> MIQKMALDEFDSLGDKVIEGYQLTDNDLRTLLSLESKEGLERLYSAARKVRDHYFGNRVFLNCFIYFSTYCKNQCSFCYYNCRNEINRYRLTMEEIKETCKTLKGAGFHMVDLTMGEDPYYYEDPNRFVEL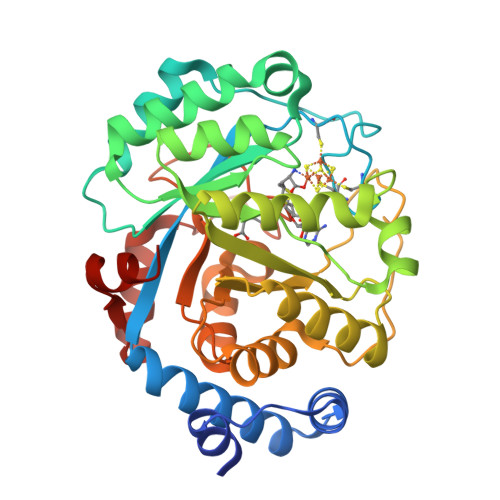VQIVKEELGLPIMISPGLMDNATLLKAREKGANFLALYQETYDTELYRKLRVGQSFDGRVNARRFAKQQGYCVEDGILTGVGNDIESTILSLRGMSTNDPDMVRVMTFLPQEGTPLEGFRDKSNLSELKIISVLRLMFPKRLIPASLDLEGIDGMVLRLNAGANIVTSILPPDSQLEGVANYDRDLEERDRDIKSVVRRLEIMGMKPARQADFEAVLGC>[6x]MNDIWWQTIGEGDCHLVLLHGWGLNAQVWDCITPQLASH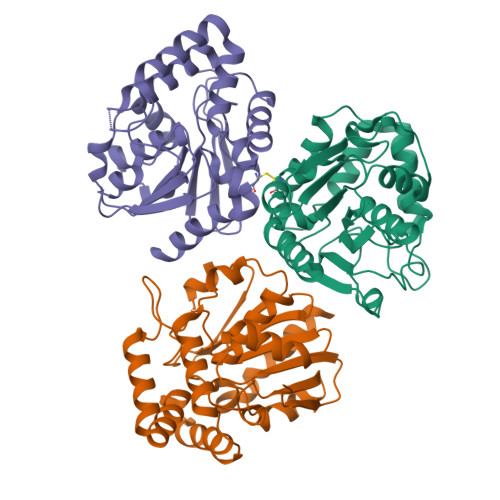FTLHLVDLPGYGRSGGFGAMSLEAMAQRVLEQAPPQAVWLGWSLGGLVASQVAIMRPERVQALVTVASSPCFAARDDWPGIKPEVLAGFQQQLSDDFQRTVERFLALQTMGTESARQDARALKQAVLSLPMPSAEALNGGLEILRTVDLRQALVRLPMPFLRLYGRLDGLVPRKIVPLLDDLWPESESILFDKAAHAPFVSHPAAFCEPLLALKTRLG> MASMKKSTENEST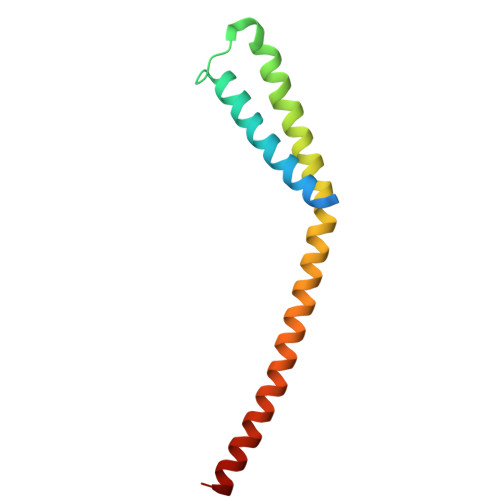NYQYKIQELRKLLKSLLLNYLELIGVLSINPDMYERKVENIRTILVNIHHLLNEYRPHQSRESLIMLLEEQLEYKRGEIREIEQVCKQVHDKLTS>[2x]SNAMPDNLALRMRPKTIDQVIGQEHLVGPGKIIRRMVEANRLSSMILYGPPGIGKTSIASAIAGTTKYAFRTFNATVDSKKRLQEISEEAKFSGGLVLLLDEIHRLDKTKQDFLLPLLESGLVIMIGATTENPFFSVTPAIRSRVQIFELEPLSNQDVKEALQIALSNPERGFDFPIELDEDALDFIATSTNGDLRSAFNSLDLAVLSTPENDEGIRHITLDIMENS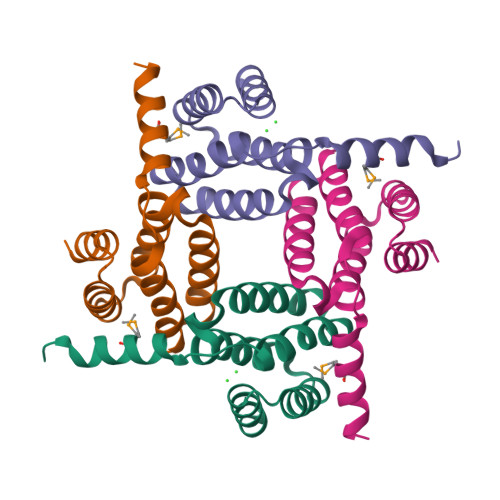LQRSYITMDKDGDGHYDVLSALQKSIRGSDVDASLHYTARLIEAGDLPSLARRLTVIAYEDIGLANPEAQIHTVTALDAAQKIGFPEARILIANVVIDLALSPKSNSAYVAMDKALADLKTSGHLPIPRHLRDGHYSGSKELGNAQDYLYPHNYPGNWVKQDYLPEKIRNHHYFQAEDTGKYERALAQRKEAIDRLRKI> RGLASKKTTTVGVIIPDISNIFYAELARGIEDIATMYKYNIILSNSDQNQDKELHLLNNMLGK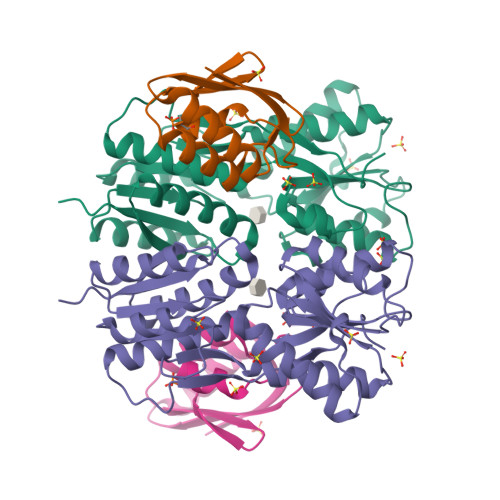QVDGIIFMSGNVTEEHVEELKKSPVPVVLAASIESTNQIPSVTIDYEQAAFDAVQSLIDSGHKNIAFVSGTLEEPINHAKKVKGYKRALTESGLPVRDSYIVEGDYTYDSGIEAVEKLLEEDEKPTAIFVGTDEMALGVIHGAQDRGLNVPNDLEIIGFDNTRLSTMVRPQLTSVVQPMYDIGAVAMRLLTKYMNKETVDSSIVQLPHRIEFRQSTK;> MAQKTFTVTADSGIHARPATTLVQAASKFDSDINLEFNGKTVNLKSIMGVMSLGIQKGATITISAEGSDEADALAALEDTMSKEGLGE> GPTGMGNRGMEDLIPLVNRLQDAFSAIGQNADLDLPQIAVVGGQSAGASSVLENFVGRDFLPRGSGIVTRRPLVLQLVNATTEYAEFLHCK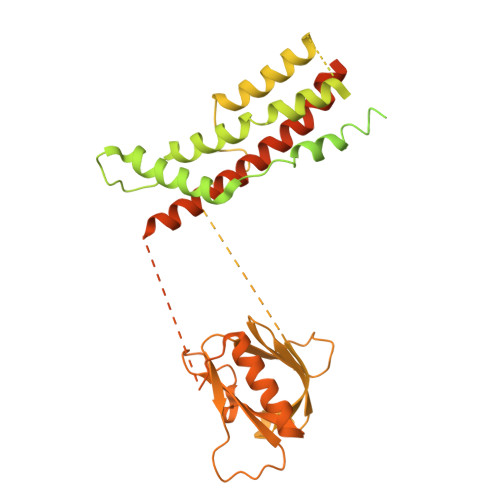GKKFTDFEEVRLEIEAETDRVTGTNKGISPVPINLRVYSPHVLNLTLVDLPGMTKVPVGDQPPDIEFQIRDMLMQFVTKENCLILAVSPANSDLANSDALKVAKEVDPQGQRTIGVITKLDLMDEGTDARDVLENKLLPLRRGYIGVVNRSQKDIDGKKDITAALAAERKFFLSHPSYRHLADRMGTPYLQKVLNQQLTNHIRDTLPGLRNKLQSQLLSIEKEVEEYKNFRPDDPARKTKALLQMVQQFAVDFEKRIEGSGDQIDTYELSGGARINRIFHERFPFELVKMEFDEKELRREISYAIKNIHGIRTGLFTPDMAFETIVKKQVKKIREPCLKCVDMVISELISTVRQCTKKLQQYPRLREEMERIVTTHIREREGRTKEQVMLLIDIELAYMNTNHEDFIGFANAQQRSNQMNKKKTSGNQDEILVIRKGWLTINNIGIMKGGSKEYWFVLTAENLSWYKDDEEKEKKYMLSVDNLKLRDVEKGFMSSKHIFALFNTEQRNVYKDYRQLELACETQEEVDSWKASFLRAGVYPERVGDKEKASETEENGSDSFMHSMDPQLERQVETIRNLVDSYMAIVNKTVRDLMPKTIMHLMINNTKEFIFSELLANLYSCGDQNTLMEESAEQAQRRDEMLRMYHALKEALSIIGNINTTTV> MNTGSFFINHEHDWQDVEPGIQRKIVAHTPDLMAVCVKFDRGAVGTPHQHERHDQIGYVVQGAFEVELEGEKRRLSPGDAFVAPHHTMHGAVALEPDSLVIDLFSPRRDDMLKS;>MNTGSFFINDEHDWQDVEPGIQRKIVAHTPDLMAVCVKFDRGAVGTPHQHERHDQIGYVVQGAFEVELEGEKRRLSPGDAFVAPHHTMHGAVALEPDS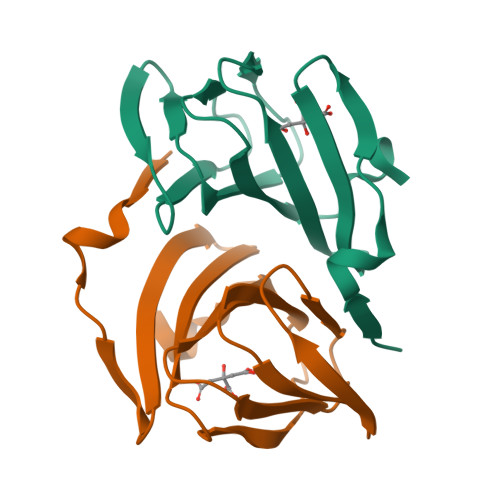LVIDLFSPRRDDMLKS[3x];> HHHHHH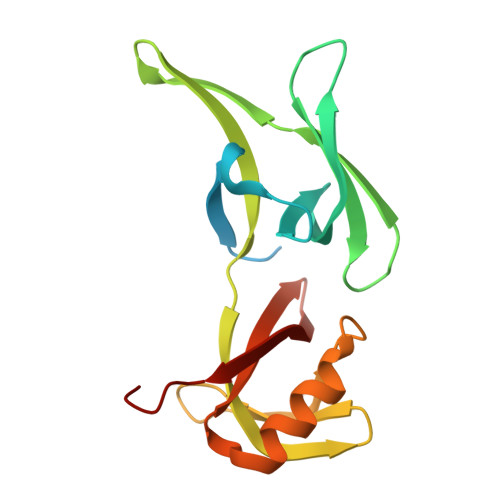> MGYYDDDAHGHVEADAAPRATTGTGTGSASQTVTIPCHHIRLGDILILQGRPCQVIRISTSAATGQHRYLGVDLFTKQLHEESSFVSNPAPSVVVQTMLGPVFKQYRVLDMQDGSIVAMTETGDVKQNLPVIDQSSLWNRLQKAFESGRGSVRVLVVSDHGREMAVDMKVVHGSRL>MAKDKEFQVLFVLTILTLISGTIFYSTVEGLRPIDALYFSVVTLTTVGETPPPQTDFGKIFTILYIFIGIGLVFGFIHKLAVNVQLPSILSNLVPR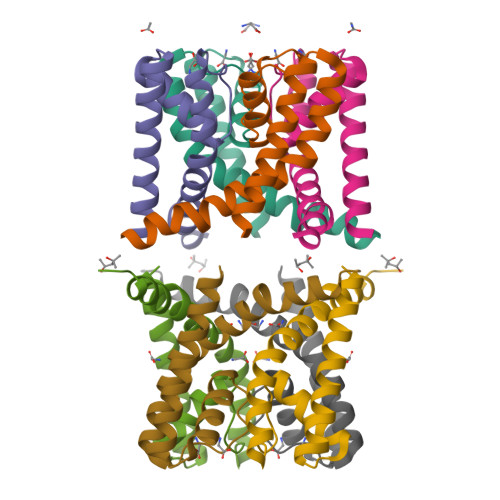[2x]> MIALGLGLGLAANGGPALRRYAVNGVAPVAVLDFERHFLSHPLALTRATSATYADALRAVQTAPADTPRYDYSTGKRALLLEASATNLLPNSAQFEAASWGKTRASVLANAALAPNGTMTADKLVEDTSNNSHFVA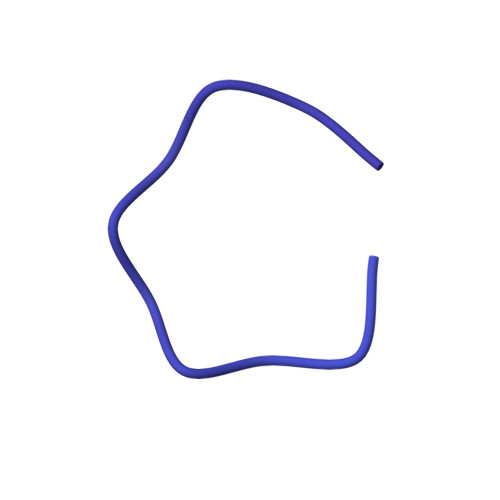RTGTQIAAGTSVTASIFVKAAERRWFALVTADSANAFRTTYFDLQTGTLGVVSQGAAGHVAQIVAAGNGWYRCSVTQTQAASGNFNFYPSVASANGATSYPGDGASGLYLWGAQLEAGAAVSSVIPTEAAAVTRAADLASVAVAAGSYDLRRVDAAGTAVTKGVAHPGGALTIGAGSLYLLSLFPAGAL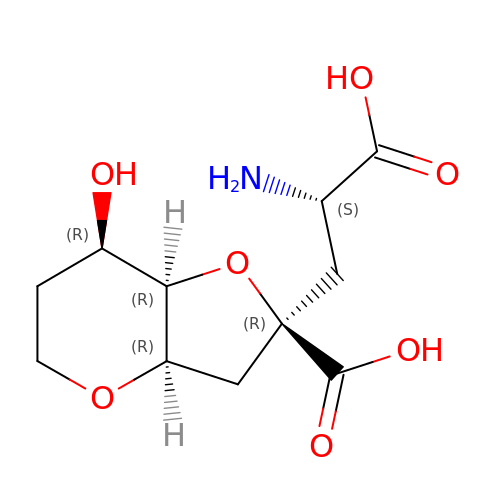(2R,3aR,7R,7aR)-2-[(2S)-2-amino-3-hydroxy-3-oxo-propyl]-7-hydroxy-3,3a,5,6,7,7a-hexahydrofuro[4,5-b]pyran-2-carboxylic acid | C11 H17 N O7 | KHYCZTHJICFSLU-XMURUDDGSA-N>MPLSVAVVGAGPRGTSVLERLCASAPELLAPGVRLTVHVVDPAPPGPGRVWRTAQSEDLLMNTVASQVTLFTDESVNCSGPILAGPSLHEWADGAIGPDDYPTRALYGRYLEWVFARTLRHAPPSVRVETHRARAVRLDDAADGRQHLALDNGRTLTGLSAVVLAQGHLPVRPSAAVLRDTEHADRHALRHIPPANPADVDLTVISPGEPVLLRGLGLNFFDHMALLTTGRGGTYVREDGVLRYVPSGREPRVYAGSRRGLPYQARGDNAKGPYGRHLPEVLTPEAVSAFRKRADSGEAPDFLRDIWPLVAKEVETVYYTALVRHPDFAPRYLSLPYGDPQEAELLAEFGVDADARWDWERVSRPYAQREFAHRGEWRQWLLGYLRADAAEALRGNVDGPLKAALDVLRDLRNELRLVVDHRGLRGDSRRDHLDRWYTPLNAFLSIGPPRRRIEELTALLEAGVVEVLGPRLEVTREDGAWLARSPDVPGSAVRVTTLIEARLPEPDLGQTADALLAHLRETGQCRAHVVDGYTTGGIDVSARPYHLVDREGVAHPRRFAFGVPTEGVHWVTAAGARPGVDSVTLSDADAVARAVLRVAGQ[2x]

FzmM and CreE catalyze the triple N-hydroxylation of L-aspartate to nitrosuccinate. The crystal structure of Streptomyces sp. V2 L-aspartate N-hydroxylase outlines a characteristic helical domain wedged between two dinucleotide-binding domains. Together with NADPH and FAD, a cluster of conserved arginine residues forms the catalytic core at the domain interface. The Lineweaver-Burk plot of the initial rates revealed a pattern of lines intercepting on the horizontal axis, suggestive of a ternary complex mechanism. Thus, Streptomyces sp. V2 L-aspartate N-hydroxylase operates as a typical class B flavoenzyme monooxygenase: it is a single-component enzyme that binds simultaneously FAD and NADPH and retains the pyridine nucleotide coenzyme throughout the catalytic process.

The enzyme was originally crystallized in conditions where the sole precipitant in the reservoir solution was ammonium sulfate. Expectedly, the protein structure is populated with sulfate ions. Two of these sulfates were found juxtaposed to the FAD and embedded by an arginine-rich site, establishing H-bond interactions with Arg266, Arg409, Arg412, Asn413, and Arg416. Notably, these residues belong to the helical substrate-binding domain. Being negatively charged molecules, we speculated that these ions occupy the putative position of the substrate and therefore inhibit the protein. Consistently, we found that the enzyme loses 50% of its activity already at 5 mM SO42- and becomes completely inhibited at 10 mM concentration. Interestingly, this effect is specific for sulfate because chloride (up to 100 mM) and phosphate (up to 50 mM) salts did not affect the enzyme. This finding highlighted the bound sulfate ions as likely substrate mimics and the associated Arg cluster as the putative site for L-aspartate binding. The crystal structure of the enzyme with NADP+ was hence solved at 2.5 Å resolution. The active site is in a cleft at the interface of the three domains and both FAD and NADP+ are clearly defined by the electron density. We noticed a difference in the conformation of this side chain between the sulfate and L-aspartate bound structures. Its side chain is oriented “inwards” in the sulfate complex to partially occupy the catalytic site.>ENIEETITVMKKLEEPRQKVVLDTAKIQLKE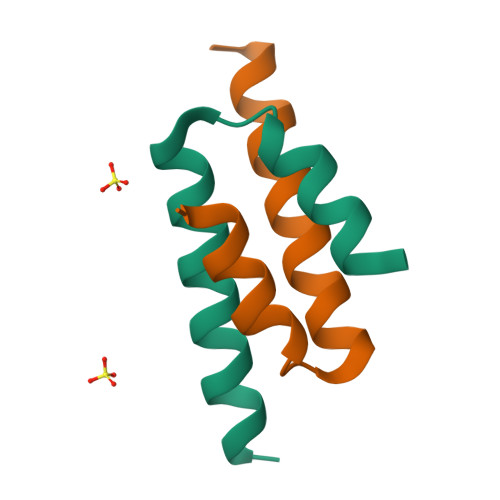QDEQ[6x]>GPGPEDWLSLLLKLEKNSVPLSDALLNKLIGRYSQAIEALPPDKYGQNESFARIQVRFAELKAIQEPDDARDYFQMARANCKKFAFVHISFAQFELSQGNVKKSKQLLQKAVERGAVPLEMLEIALRNLNLQKKQLLSEEEKKNLSASTVLTAQ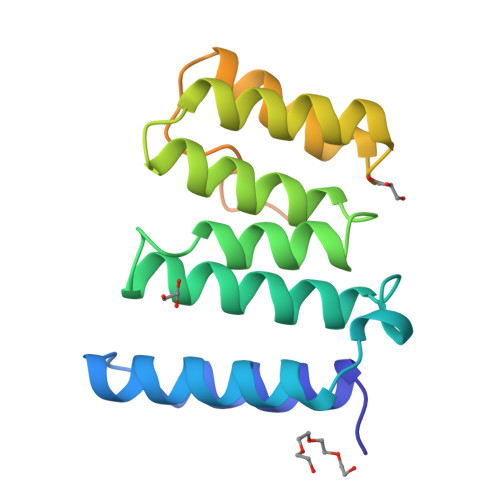ESFSGSLGHLQNRNNSCDSRGQTTKAR[4x]>[2x]MSLKDMIDSIEQFAQTQADFPVYDCLGERRTYGQLKRDSDSIAAFIDSLALLAKSPVLVFGAQTYDMLATFVALTKSGHAYIPVDVHSAPERILAIIEIAKPSLIIAIEEFPLTIEGISLVSLSEIESAKLAEMPYERTHSVKGDDNYYIIFTSGTTGQPKGVQISHDNLLSFTNWMIEDAAFDVPKQPQMLAQPPYSFDLSVMYWAPTLALGGTLFALPKELVADFKQLFTTIAQLPVGIWTSTPSFADMAMLSDDFCQAKMPALTHFYFDGEELTVSTARKLFERFPSAKIINAYGPTEATVALSAIEITREMVDNYTRLPIGYPKPDSPTYIIDEDGKELSSGEQGEIIVTGPAVSKGYLNNPEKTA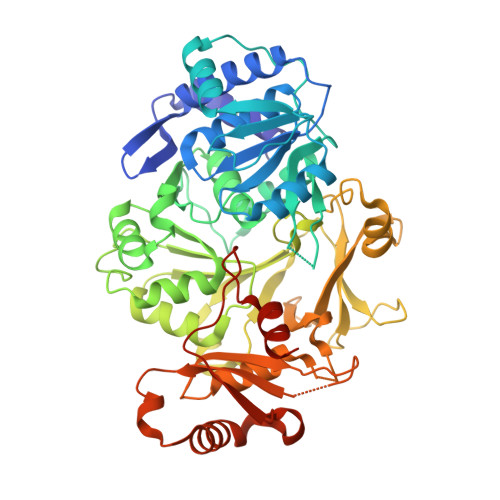EAFFTFKGQPAYHTGDIGSLTEDNILLYGGRLDFQIKYAGYRIELEDVSQQLNQSPMVASAVAVPRYNKEHKVQNLLAYIVVKDGVKERFDRELELTKAIKASVKDHMMSYMMPSKFLYRDSLPLTPNGKIDIKTLINEVNNREGHHHHHH> MVLPDIKKGKDMINILPFEIISRNTKTLLITYISSVDITHEGMKKVLESLRSKQGIISEYLLDKLLDESLIDKDKGKEFLITTGVINKTKTSPLWVNSVIISDVPHLFSNAREQWKCDGVF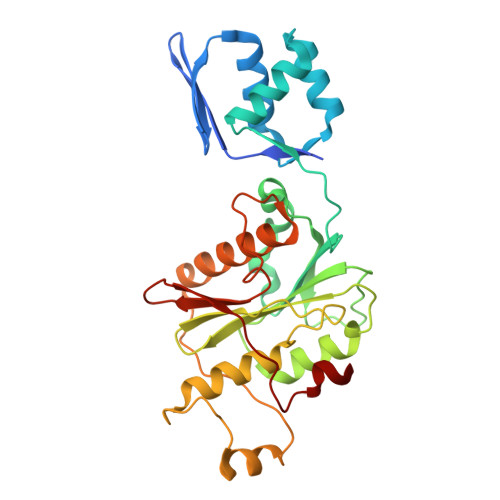VSHIIDIKDNNINVSDSTLIWLHLENYHSDIVKRIYSKFESNPGVAFIQSYYLKESFRIDGVYSPDLGTPCHFCHIERWLSREEKSFRRNEMSWANLLQLLKKYQMTLPALALGESERGFSYHLIKRRLQELTGTSLVKSHVDNFMSSVSADLITCILCKEPVIHWQACSCLER>EKIVVPVQQLDPQNGNKDVGTVEITESAYGLVFTPK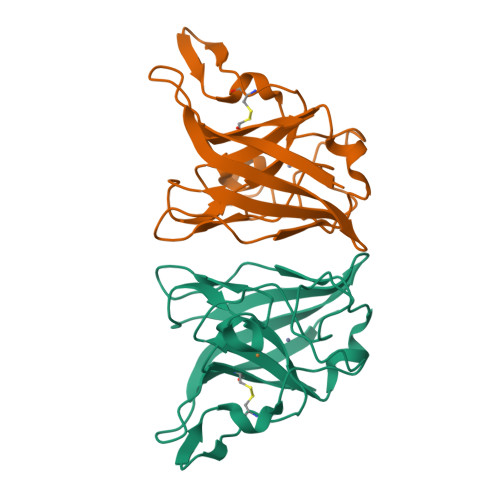LHDLAHGLHGFHIHEKPSCEPKEKDGKLVAGLGAGGHWDPKQTQKHGYPWSDDAHMGDLPALFVMHDGSATTPVLAPRLKKLAEVKGHSLMIHAGGDNHSDHPAPLGGGGPRMACGVIK[2x]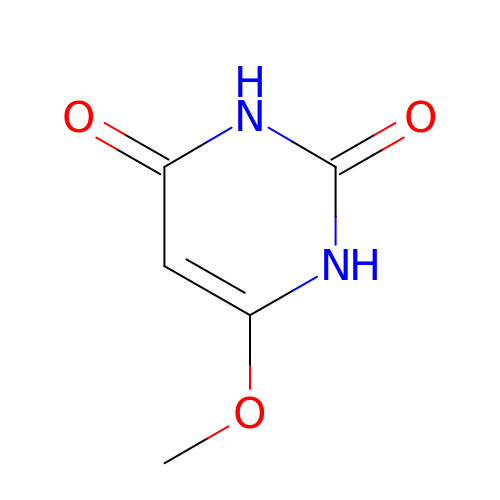6-methoxy-1H-pyrimidine-2,4-dione | C5 H6 N2 O3 | SWNDNOHEVRPIDI-UHFFFAOYSA-N> MGQLRKLLLPGLLSVTLLSGCGMGSGSKTEQPKLDYQSRSHRLIKLEVPPDLNNPDQGNLYRLPA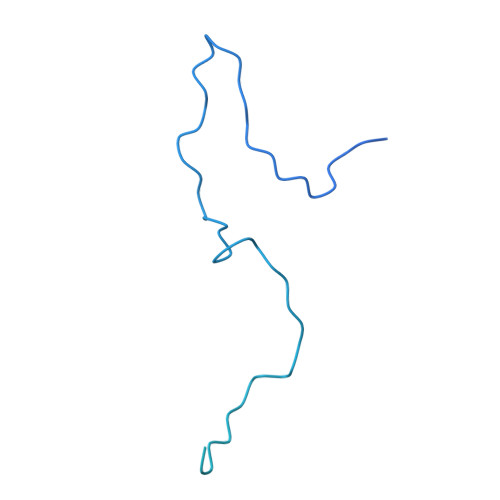GSGAVRASDLEKRRTPAVQQPADAEVLKSVKGVRLERDGSQRWLVVDGKSPAEIWPLLKAFWQENGFDIESEEPAIGQMETEWAENRAKIPQDSLRRLFDTVGLGGIYSTGERDKFIVRIEQGKNGVSDIFFAHKAMKEVYGDKNKDTTMWQPSASDPNLEAAFLTRFMQYLGVDGRQAENALAKKPTLPAANEMARIEGKSLIVFGDYGRNWRRTGLALDRIGLTVVGQNTERHAFLVQKAPNESNAVTEQKPGLFKRLLGKGKAEKPAEQPELIVYAEPVADGSRIVLLNKDGSAYAGKDASALLGKLHSELR> MAIPKIASYQ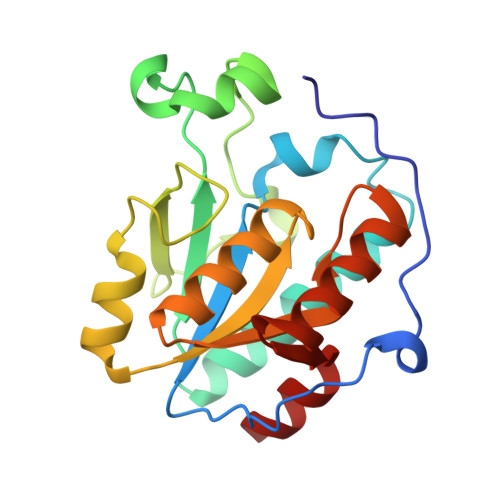VLPLESFPTNKVDWVIDPKKSVVLVHDLQAYFLNFFDKTLSPVPELLRNVNKVTESARSAGIPVVYTAQPANQDPNERALLTDFWGVGLTQDTEIVPEVSPQPEDIQYTKWRYSAFKKTPLLEWMKEEQRDQLVIVGVYGHIGILSTALDAFMLDIKPFVIGDAIADFSKEDHMNTLKYVASRSGSVKSVDEFIDSVT>ADTTGRAYNLTWKSTNFKTILEWEPKSIDHVYTVQISTRLENWKSKCFLTAETECDLTDEVVKDVGQTYMARVLSYPARNGNTTGFPEEPPFRNSPEFTPYLDTNLGQPTIQSFEQVGTKLNVTVQDARTLVRRNGTFLSLRAVFGKDLNYTLYYWRASSTGKKTATTNTNEFLIDVDKGENYCFSVQAVIPSRKRKQRSPESLTECTSREQGRAREMF[2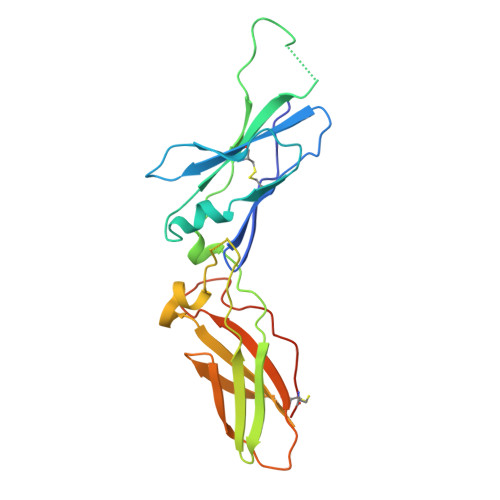x]>[2x]MSMSKQVLKEDMKMTYHMDGSVNGHYFTIEGEGTGNPFKGQQTLKLRVTKGGPLPFAFD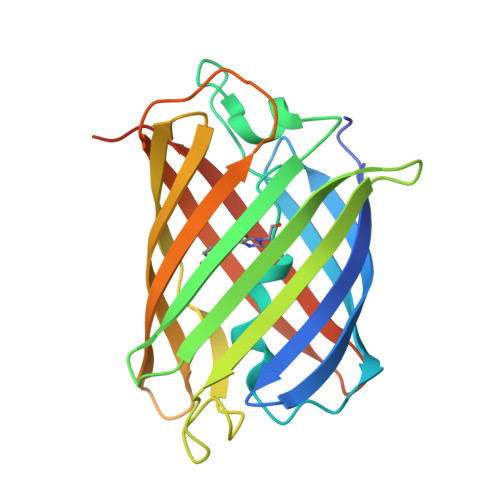ILSPTFTYGNRVFTDYPEDMPDYFKQSLPEGYSWERTMMYDDGASATASARISLDKNGFVHKSTFHGENFPANGPVMKKKGVNWEPSSETITASDGILKGDVTMFLVLEGGQRLKALFQTTYKANKVVKMPPRHKIEHRLVRSEDGETIQLQEHAVAKYFTEGSHHHHHH>GAMNAQAEEFKKYLETNGIKPKQFHKKELIFNQWDPQEYCIFLYDGITKLTSISENGTIMNLQYYKGAFVIMSGFIDTETSVGYYNLEVISEQATAYVIKINELKELLSKNLTHFFYVFQTLQKQVSYSLAKFNDFSINGKFGSICGQLLILTYVYGKETPD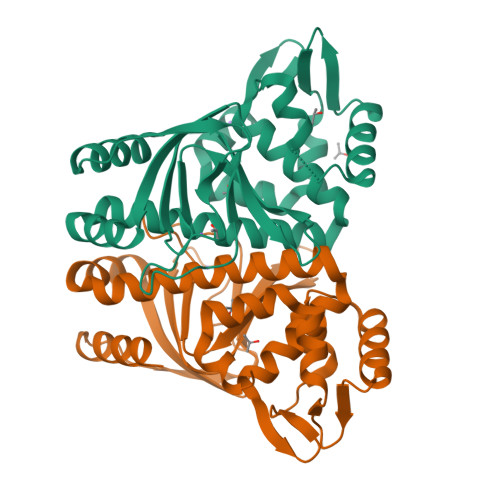GIKITLDNLTMQELGYSSGIAHSSAVSRIISKLKQEKVIVYKNSCFYVQNLDYLKRYAPKLDEWFYLACPATWGKLN[2x]> GDNQDRTVANTQPSGPSNSKEIPALTAVETGHTSQVDPSDTLQTRHVVNFHSRSESTVENFMGRAACVFMDQYKLNGEETSTDNFAVWTINVREMAQLRRKCELFTYMRFDIEMTMVITSCQDQGTQLEQDMPVLTHQIMYVPPGGPIPAKVDSYEWQTSTNPSVFWTEGNAPARMSIPFISVGNAYSLFYDGWSHFTQDGTYGYTTLNAMGKLFVRHVNKSSPHQITSTIRVYFKPKHIKAWVPRPPRLCPYINKGDVNFVVTEVTDARKSITDTP;> SPSAEECGYSDRVRSMTLGNSTITTQESANVV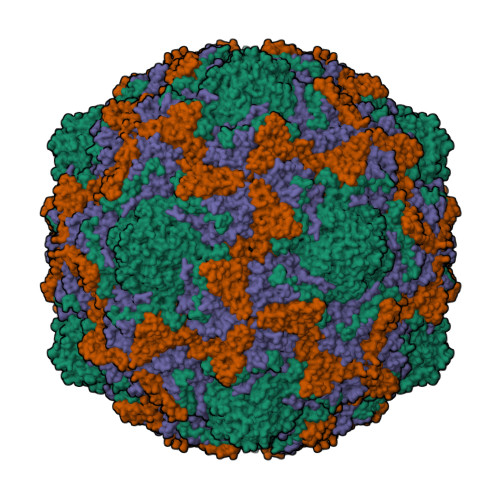VGYGEWPSYLSDKEATAEDQPTQPDVATCRFYTLESVQWEKSSPGWWWKFPEALKNMGLFGQNMHYHYLGRAGYTIHVQCNASKFHQGCLLVVCVPEAEMGCADTSTTFPATELTTEEEPHVFTSDSITGKKVQAAVCNAGMGVGVGNLTIFPHQWINLRTNNSATIVMPYINSVPMDNMFRHYNFTLMIIPFAPLNFNEGATAYVPVTVTIAPMYAEYNGLRLASTQ;> GVPVLNTPGSTQFLTSDDFQSPSAMPQFDETPEMHIPGEVRNLMEMAEVDSVVPVNNITGKTKSMEAYQIAVGTGNTDKTKPIFSFQMDPGYSSVLKRTLLGEMLNYYAHWSGSVKLTFLFCGSAMATGKLLISYSPPGASVPSSRKDAMLGTHIIWDIGLQSSCVLCVPWISQSHYRMVQQDPYTSAGYITCWYQTNIVVPPGAPTSCDVLCFASACNDFSVRLLRDTPFMAQPGKLQ;> MGAQVSTQKTGAHETSLNAKGNSIIHYTNINFYKDAASSASNRQELQQDPGKFTDPVKDLMVKTLPALN>MKMLEQLEKKLGYTFKDKSLLEKALTHVSYSKKEHYETLEFLGDALVNFFIVDLLVQYSPNKREGFLSPLKAYLISEEFFNLLAQKLELHKFIRIKRGKINETIIGDVFKALWAAVYIDSGRDANFTRELFYKLFKEDILSAIKEGRVKKDYKTILQEITQKRWKERPEYRLISVEGPHHKKKFIVEAKIKEYRTLGEGKSKKEAEQRAAEELIKLLEESE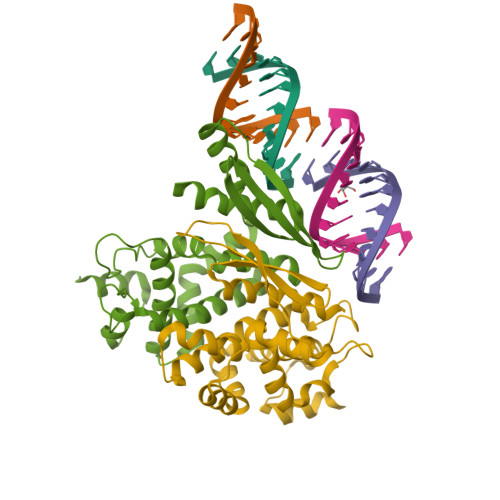[2x]>[2x]SQDIVDFSQHPWKAPGPNDLRSPCPGLNTLANHGFLPRNGRNITIPMIVQAGFDGYNVQPDILILAAKVGLLTSPEPDTFTLDDLKLHGT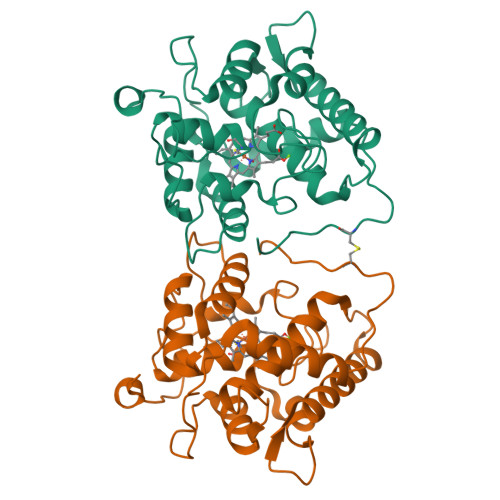IEHDASLSREDFALGDNLHFNEAIFNTLANSNPGSDVYNITSAGQVLKDRLADSLARNPNVTNTGKEFTIRTLESAFYLSVMGNATTGEAPKNFVQIFFREERLPIEEGWKRSTTPITSDTLNPIAGQISEASNWKPNPDQCPWIVLSPNL(1S,2S,3R,4S,5S)-5-[(1,3-dihydroxypropan-2-yl)amino]-1-(hydroxymethyl)cyclohexane-1,2,3,4-tetrol | C10 H21 N O7 | 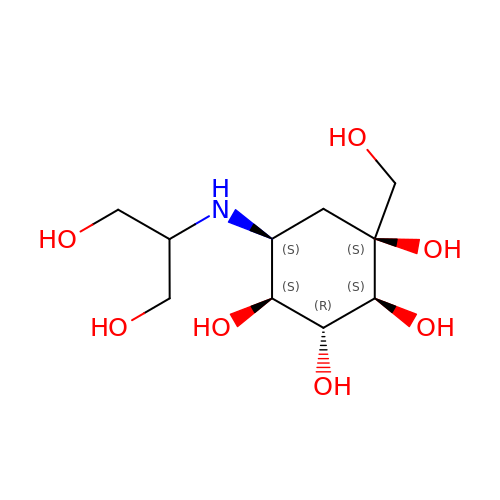FZNCGRZWXLXZSZ-CIQUZCHMSA-N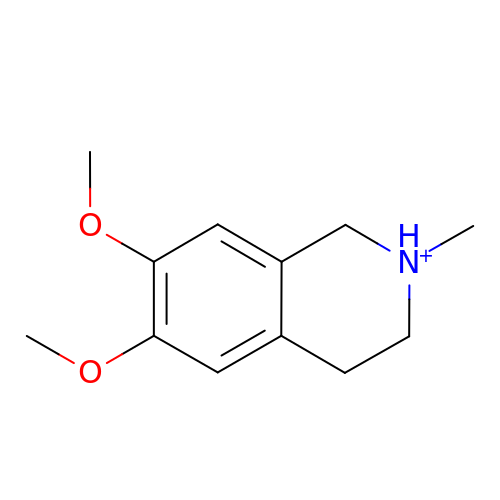6,7-dimethoxy-2-methyl-1,2,3,4-tetrahydroisoquinolin-2-ium | C12 H18 N O2 | TXPPKWZEHFNZOE-UHFFFAOYSA-O(3S,4R,5R,6S)-1-(2-hydroxyethyl)azepane-3,4,5,6-tetrol 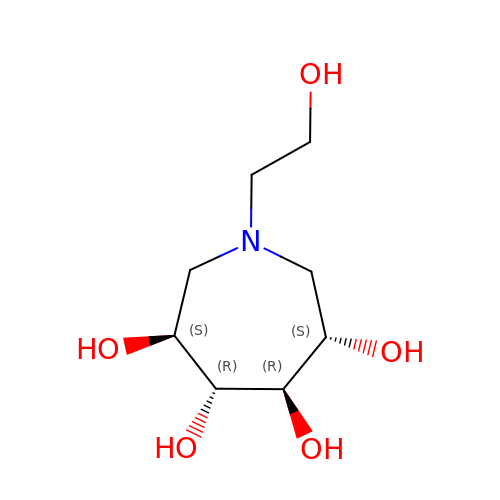| C8 H17 N O5 | VWGJHYNWDXVPIU-RULNZFCNSA-N>[7x]MSLAHTAAEYMLSDALLPDRRGPRLKG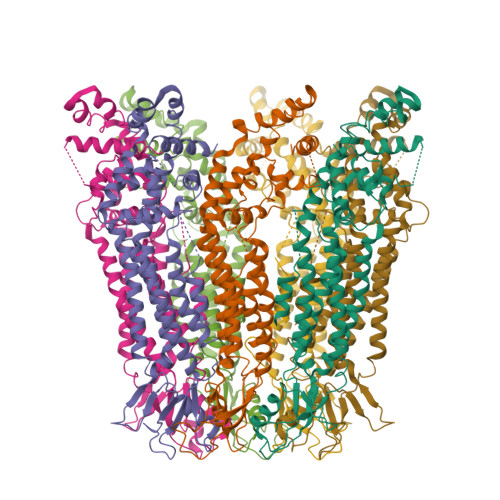LRLELPLDRIVKFVAVGSPLLLMSLAFAQEFSSGSPISCFSPSNFSIRQAAYVDSSCWDSLLHHKQDGPGQDKMKSLWPHKALPYSLLALALLMYLPVLLWQYAAVPALSSDLLFIISELDKSYNRSIRLVQHMLKIRQKSSDPYVFWNELEKARKERYFEFPLLERYLACKQRSHSLVATYLLRNSLLLIFTSATYLYLGHFHLDVFFQEEFSCSIKTGLLSDETHVPNLITCRLTSLSIFQIVSLSSVAIYTILVPVIIYNLTRLCRWDKRLLSVYEMLPAFDLLSRKMLGCPINDLNVILLFLRANISELISFSWLSVLCVLKDTTTQKHNIDTVVDFMTLLAGLEPSKPKHLTNSACDEHP>[2x]AESTLGAAAAQSGRYFGTAIASGKLGDSAYTTIASREFNMVTAENEMKIDATEPQRGQFNFSAGDRVYNWAVQNGKQVRGHTLAWHSQQPGWMQSLSGSTLRQAMIDHINGVMGHYKGKIAQWDVVSHAFSDDGSGGRRDSNLQRTGNDWIEVAFRTARAADPAAKLCYNDYNIENWTWAKTQGVYNMVRDFKQRGVPID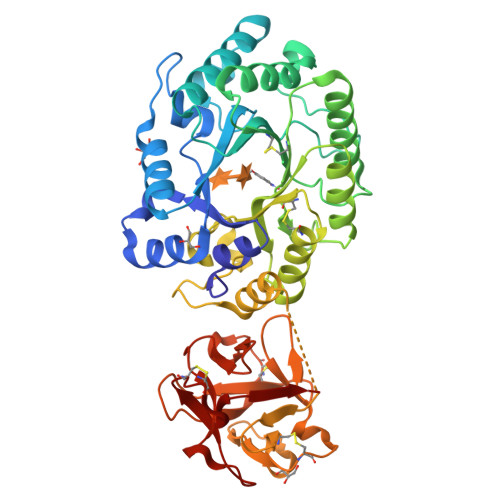CVGFQSHFNSGSPYNSNFRTTLQNFAALGVDVAITELDIQGASSSTYAAVTNDCLAVSRCLGITVWGVRDTDSWRSGDTPLLFNGDGSKKAAYTAVLNALNGGSSTPPPSGGGQIKGVGSGRCLDVPNASTTDGTQVQLYDCHSATNQQWTYTDAGELRVYGDKCLDAAGTGNGTKVQIYSCWGGDNQKWRLNSDGSIVGVQSGLCLDAVGGGTANGTLIQLYSCSNGSNQRWTRT>[2x]MYIPKHFAVNDPDVAYQVIEENSFATLV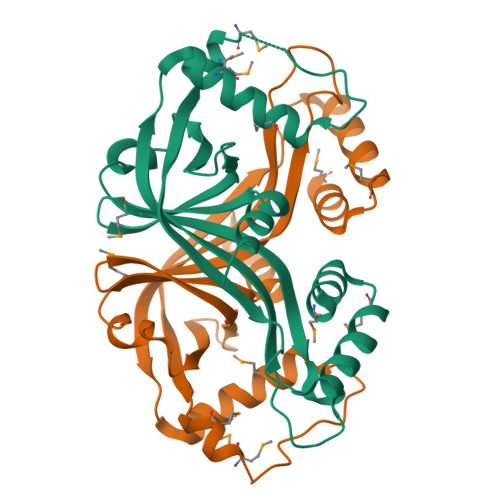SMHQRELFATHLPLLLDREKTCLYGHFARSNPQWNDIQHQTVLAIFHGPHCYISPSWYETNQAVPTWNYVAVHVYGNVELINDQGEVMQSLHDMVEKYEAPGSRYQLSEVDAGMLSGMNKGIQAFKIIIKRIEGKAKLSQNHPAHRQERIIKQLEQMPFENEKRIASLMKKQRQ>MAPYTVVYFPVRGRCAALRMLLADQGQSWKEEVVTVETWQEGSLKASCLYGQLPKFQDGDLTLYQSNTILRHLGRTLGLYGKDQQEAALVDMVNDGVEDLRCKYISLIYTNYEAGKDDYVKALPGQLKPFETLLSQNQGGKTFIVGDQISFADYNLLDLLLIHEVLAPGCLDAFPLL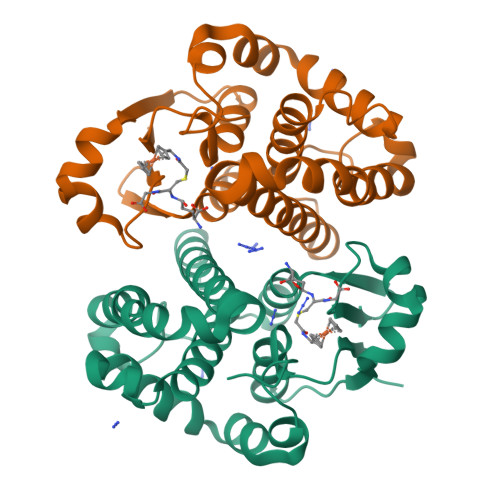SAYVGRLSARPKLKAFLASPEYVNLPINGNGKQ[2x]>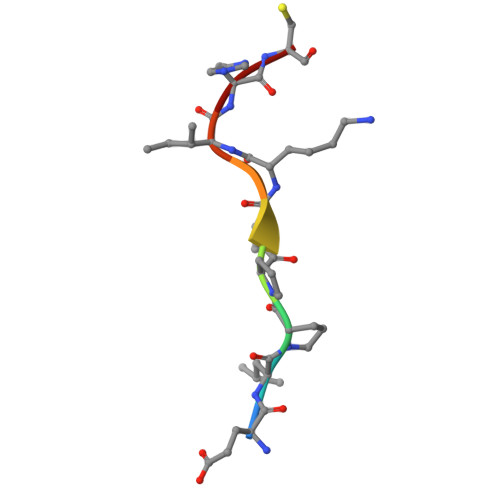 ELPPVKIHC> GASLEHHHHHHENLYFQSGTRWAVLV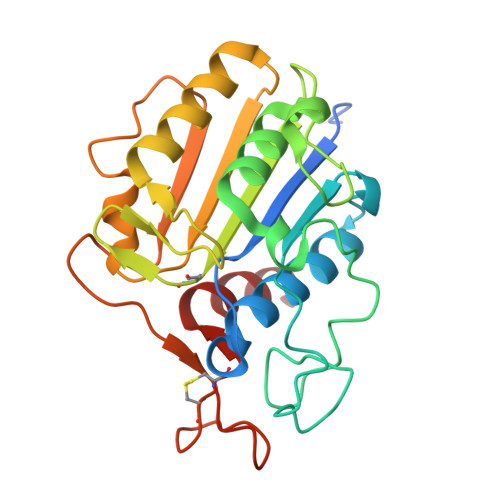AGSSGYWNYRHQADICHAYQLLRKGGLKEENIVVFMYDDIANNYENPRPGTIINSPHGKDVYQGVPKDYTGDDVNVDNLFAVILGDKTAVKGGSGKVVDSGPNDHIFIFYSNHGGPGVLGMPTSPYLYANDLNDVLKKKHALGTYKSLVFYLEACESGSIFEGLLPEGLNIYATTASNAEESSWGTYCPGEEPSPPPEYETCLGDLYSVAWMEDSGMHN> MSALQAVK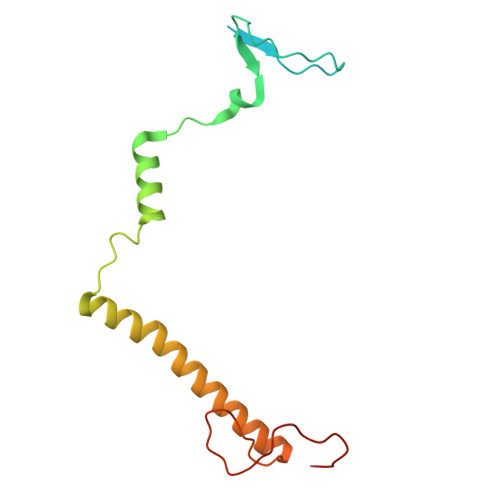NLTTRMRPFAFQQIRKASNSSRIAGDTTGKYTPNIFSPETPMDRSFSHVPKNPFWEAWVFRRDNIQREFVWTWQTIFDLATFVGGLYVAMYATASFCSRQNDKRNGYPERNYYFSDSKSNFVIPDEREFY>MYGSKTFIKYVSGIPDYFKQSFPEGFTWERTTTYEDGGFLTAHQDTSLDGDCLVYKVKILGNNFPADGPVMQNKAGGWEPSCEILYEVDGVLCGQSLMALKCPGGRHLNCRLHTTYRSKKPASALKMPEFHFEDHRIEVKEVQKGKHYEQYEAAVARYCDAAPSKLGHH[4x];>MASLLTETMPFRMTMEGTVNGHHFKCTGKGEGNPFEGTQDMKIEVIEGGPLP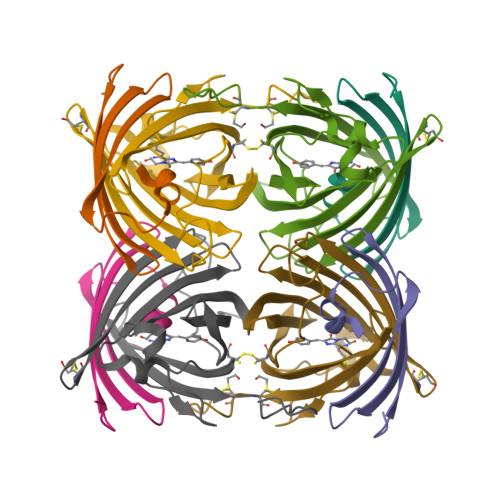FAFDILSTSC[4x]>[2x]ALLTAETFRLQFNNKRRLRRPYYPRKALLCYQLTPQNGSTP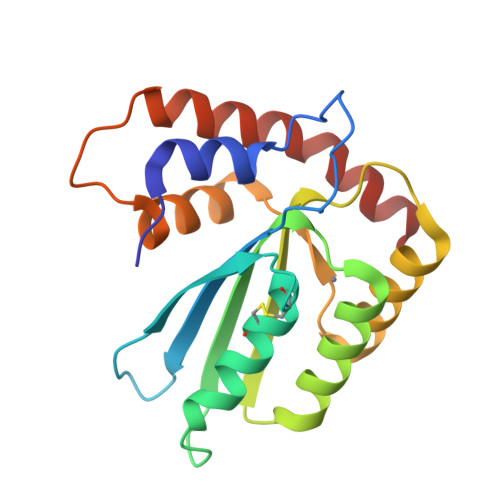TRGYFENKKKCHAAICFINEIKSMGLDETQCYQVTCYLTWSPCSSCASELVDFIKAHDHLNLRIFASRLYYHASKPQQDGLRLLSQEGVPVEVMGFPEFADCWENFVDHEKPASFNPYKMLEELDKNSRAIKRRLDRIKS>MPRMTAVEAAVHVMRLEGVDTAFGVPGAAINPLYAALRKVGGVNHILARHVEGASHMADGYTRAKFGNIGVCIGTSGPAGTDMITGLYAAIADSVPILCITGQAPRARLYKEDFQAVDIESIAKPVTKMAVTVREPALVPYVFQQAFHVMRSGRPGPVLIDLPFDVQMTEIEFDPETYAPLPIYKPLATRAQVEKAMTMLNASERPLLVSGGGVIGADASDLLVQFAELTGVPVIPTLMGWGSIPDDHPLMVGMVGLQTSQRYGNANLLASDFVMGIGNRWANRHTGGLDVYTEGRKFVHVDIEPTQIGRVFGPDYAIVSDAKAALQLFVEVAREWRAAGKLKDRGEWAESCRERKRTMLRKTHYDNVPIKPQRVYEEMNKAFGRDVTYVTTIGLSQIAGGQFLHVYKPRHWINAGQAGPLGWTVPAALGVAAAKPGAEIVALSGDYDFQFMIEELAVGAQFNLPFIQVLVNNSYLGLIRQSQRGFDMD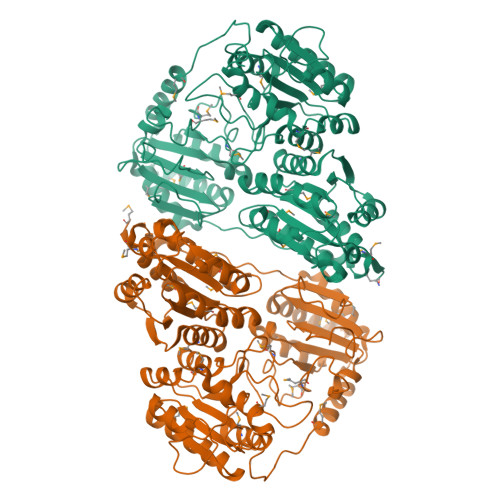YQVQLSFENINSPEVNGYGVDHLKVVEGLGCKALRVFKPDDILPAFEKARDLMQEYRVPVVVEVILERV[2x]> MAASSSGEKEKERMGGVSGMAGLGSTRERLLSALEDLEVLSRELIEMLAISRNQKLLQLEEENQVLELLIHRDGDFQELMKLALNQGKVHHEMQALEKEVEKRDSDIQQLQKQLKEAEQILATAVYQAKEKLKSIEKARKGAISSEEIIKYAHRISASNAVCAPLTWVPGDPRRPYPTDLEMRSGLLGQMNNP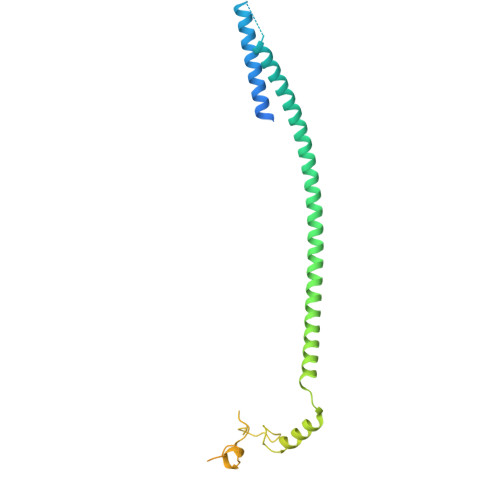STSGVNGHLPGDALAAGRLPDVLAPQYPWQSNDMSVNMLPPNHSSDFLLEPPGHNKENEDDVEVMSTDSSSSSSDSD> MCASRDDWRCARSMHEFSAKDIDGHMVNLDKYRGFVCIVTNVASQUGKTEVNYTQLVDLHARYAECGLRILAFPCNQFGKQEPGSNEEIKEFAAGYNVKFDMFSKICVNGDDAHPLWKWMKIQPKGKGILGNAIKWNFTKFLIDKNGCVVKRYGPMEEPLVIEKDLPHYFHHHHHH

The isoform GPX4 belongs to a subfamily of selenium-containing GPX enzymes and is unique in that it can also reduce hydroperoxides in complex lipids such as phospho­lipids, cholesterol and cholesteryl ester hydroperoxides, even when they are inserted into biomembranes or lipoproteins. The catalytic mechanism of the GPX reaction involves redox shuttling of this selenocysteine between the redox states selenol (Se–H) and selenenic acid (Se–OH). The catalytic site of GPX enzymes was initially suggested to consist of a catalytic triad formed by a selenocysteine, a glutamine and a tryptophan residue. This was later extended by a conserved asparagine to form a catalytic tetrad, which in human GPX4 consists of Sec46, Gln81, Trp136 and Asn137. Recently, GPX4 has been identified as a key player in ferroptosis, a non-apoptotic cell death resulting from the iron-dependent accumulation of lipid reactive-oxygen species.

In order to produce the true wild-type protein, we employed a novel approach, first described by Eaton et al., in which wild-type GPX4 was co-expressed with selenocysteine insertion sequence-binding protein 2 (SBP2) in mammalian cells on a 10–30 l scale. The protein was purified and crystallized, and the crystal structure of the wild-type form of GPX4 was determined at 1.0 Å resolution. The structure was solved by molecular replacement. In the refined structure, the active-site selenocysteine residue Sec46 was clearly defined in the electron-density map, but the difference density maps showed a strong peak at the Se atom. Reducing the occupancy of the Se atom to 0.60 removed most of the difference density. The reduced occupancy of the Se atom in the structure may therefore be owing to radiation damage, aggravated by the long exposure time that was required to achieve sufficient completeness in space group P1. At the very high resolution obtained here, many side chains needed to be modeled in alternative conformations. Additionally, one of the histidine residues of the C-terminal hexahistidine tag could be built in the electron-density maps. The apo wild-type GPX4 structure described here is very similar to previously reported mutant GPX4 structures. In the wild-type apo GPX4 structure reported here, there is only very weak difference density on the Se atom, which did not justify modeling it as an oxidized form. This difference in oxidation may be related to the tenfold higher concentration of the reducing reagent TCEP used in our study.> GAMTRKGYGESTGKIILIGEHAVTFGEPAIAVPFNAGKIKVLIEALESGNYSSIKSDVYDGMLYDAPDHLKSLVNRFVELNNITEPLAVTIQTNLPPSRGLGSSAAVAVAFVRASYDFLGKSLTKEELIEKANWAEQIAHGKPSGIDTQTIVSGKPVWFQKGHAETLKTLSLDGYMVVIDTGVKGSTRQAVHDVHKLCEDPQYMSHVKHIGKLVLRASDVIEHHKFEALADIFNECHADLKALTVSHDKIEQLMKIGKENGAIAGKLTGAGRGGSM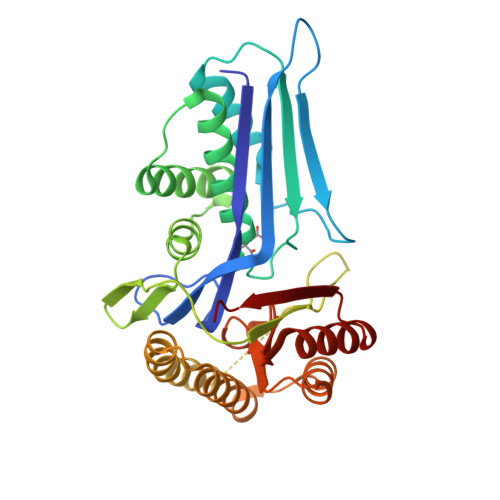LLLAKDLPTAKNIVKAVEKAGAAHTWIENLGG>[12x]SNADKSMELMKTLMEAFGPSGFEREVNAICKEYMEPYADEVVVDKLGSVTFIAKGNDRPRILMAGHTDEVGFIVSSISKE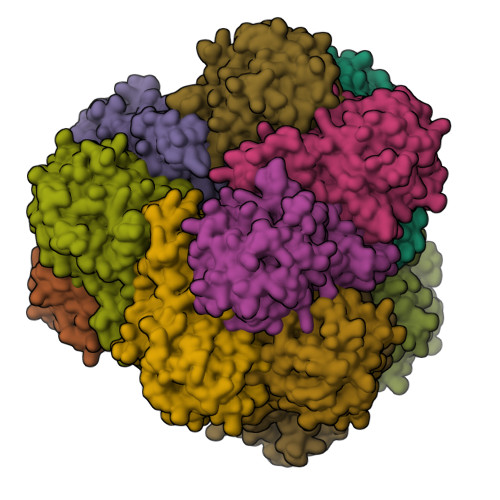GYLTFNTLGGWWSQVLLGQRVVVRTCKGMVHGIIASKPPHILPPDERKKIVEARDMFIDIGATSEEEAEESGVKVGDPIVPWSPFSVIQNGRVAMGKAFDDRIGAFVLMEAIRRMKDQGIEHPNTVYGSATVQEEVGLRGAQTTAHVVDPDVALVLEVDIAGDVPGIKPHEALTKMGKGPGLVTYDRSMIPNQPLKEFVINVAKQAQIPLQLSQMSGGGTDAGRIHMNRAGCPSVVITIPTRHIHSHVGLLSLKDTENAIRLVIELIKRLDLETVEGFT> SLMSVDPNYTEMEGKVREATNNEPWGASSTLMDQISQGTYNFREREEILSMIFRRFTEKAGSEWRQIYKALQLLDYLIKHGSERFIDDTRNSINLIRIL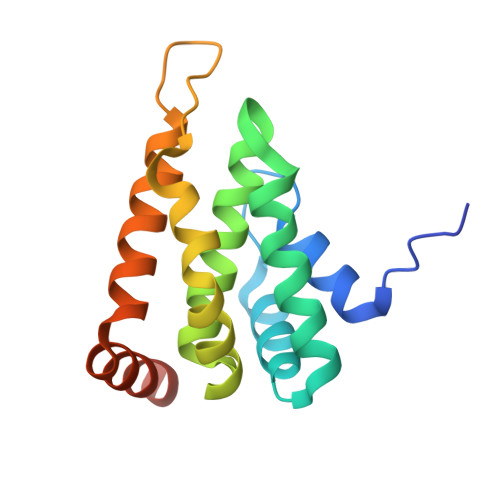ETFHYIDSQGRDQGINVRTRVKALIELLSDDNKIRAERKKARETAKKYKGV>[2x]MFQTFEGDLKWHHHNITYWIQNYSEDLPRAVIDDAFARAFALWSAVTPLTFTRVYSRDADIV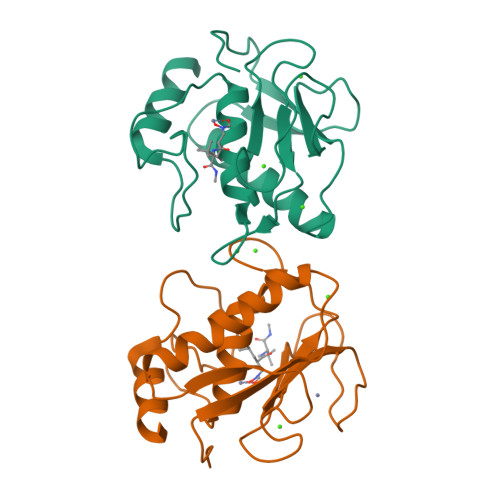IQFGVAEHGDGYPFDGKDGLLAHAFPPGPGIQGDAHFDDDELWSLGKGQGYSLFLVAAHQFGHALGLDHSSVPEALMYPMYRFTEGPPLHKDDVNGIRHLY>[2x]MSVKTKEKEMAVTILYEQDVDPKVIQGLKVGIIGYGSQGHAHALNLMDSGVDVRVGLREGSSSWKTAEEAGLKVTDMDTAAEEADVIMVLVPDEIQPKVYQEHIAAHLKAGNTLAFAHGFNIHYGYIVPPEDVNVIMCAPKGPGHIVRRQFTEGSGVPDLACVQQDATGNAW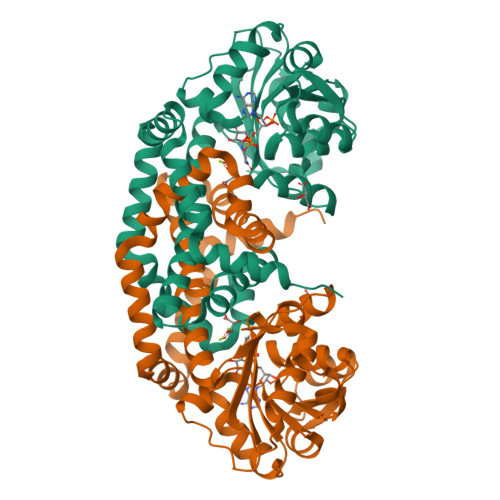DIVLSYCWGVGGARSGIIKATFAEETEEDLFGEQAVLCGGLVELVKAGFETLTEAGYPPELAYFECYHEMKMIVDLMYESGIHFMNYSISNTAEYGEYYAGPKVINEQSREAMKEILKRIQDGSFAQEFVDDCNNGHKRLLEQREAINTHPIETTGAQIRSMFSWIKKEDLEHHHHHH> GSGAMAKKEDGESTAPTPRPKILRCKCHHHCPEDSVNNICSTDGYCFTMIEEDDSGMPVVTS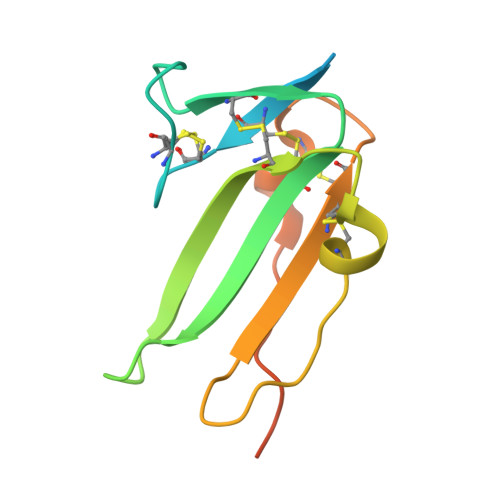GCLGLEGSDFQCRDTPIPHQRRSIECCTERNECNKDLHPTLPPLKDRDFVDGPIHHK>ANPLYQKHIISINDLSRDDLNLVLATAAKLKANPQPELLKHKVIASCFFEASTRTRLSFETSMHRLGASVVGFSDSANTSLGKKGETLADTISVISTYVDAIVMRHPQEGAARLATEFSGNVPVLNAGDGSNQHPTATLLDLFTIQETQGRLDNLHVAMVGDLKYGRTVHSLTQALAKFDGNRFYFIAPDALAMPQYILDMLDEKGIAWSLHSSIEEVMAEVDILYMTRVQKERLDPSEYANVKAQFVLRASDLHNAKANMKVLHPLPRVDEIATDV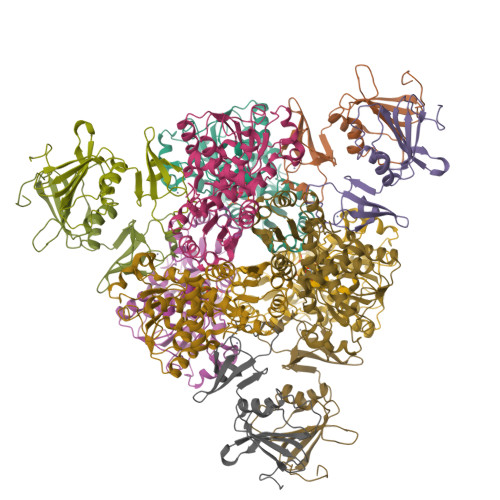DKTPHAWYFQQAGNGIFARQALLALVLNRDLVL[2x];>[2x]MTHDNKLQVEAIKRGTVIDHIPAQIGFKLLSLFKLTETDQRITIGLNLPSGEMGRKDLIKIENTFLSEDQVDQLALYAPQATVNRIDNYEVVGKSRPSLPERIDNVLVCPNSNCISHAEPVSSSFAVRKRANDIALKCKYCEKEFSHNVVLAN> ADLANGAKVFSGNCAACHMGGGNVVMANKTLKKEALEQFGMYSEEAIIYQVQHGKNAMPAFAGRLTDEQIQDVAAYVLDQAAKGWV;> ADLANGAKVFSGNCAAC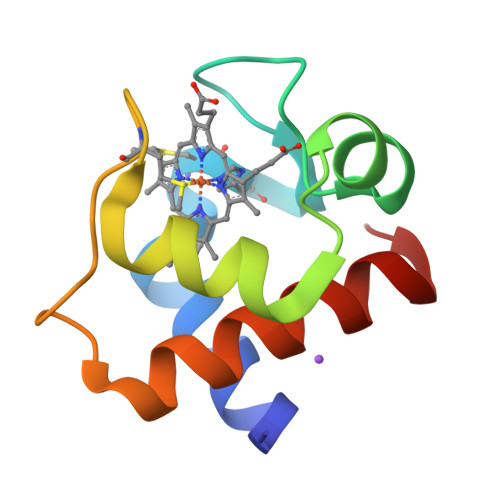HMGGGNVVMANKTLKKEALEQFGMYSEEAIIYQVQHGKNAMPAFAGRLTDEQIQNVAAYVLDQAAKGWAG;> ADLANGAKVFSGNCAACHMGGGNVVMANKTLKKEALEQFGMYSEDAIIYQVQHGKNAMPAFAGRLTDEQIQDVAAYVLDQAAKGWV(1-propan-2-ylpyrazol-4-yl)methyl 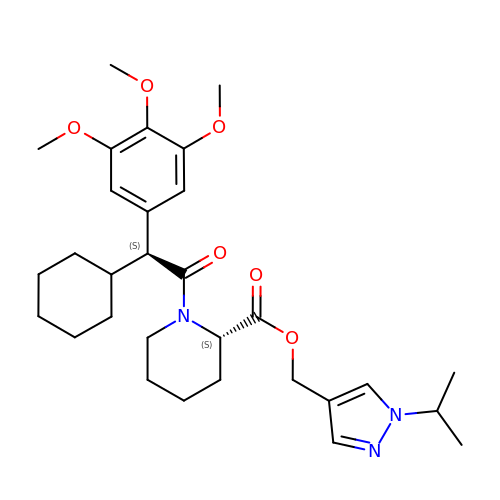(2S)-1-[(2S)-2-cyclohexyl-2-(3,4,5-trimethoxyphenyl)ethanoyl]piperidine-2-carboxylate | C30 H43 N3 O6 | UJDKLVXYTQFNCX-IGKIAQTJSA-N>MPVAGSELQYLGQIQHILRCGVRKDDRTGTGTLSVFGMQARYSLRDEFPLLTTKRVFWKGVLEELLWFIKGSTNAKELSSKGVKIWDANGSRDFLDSLGFSTREEGDLGPVYGFQWRHFGAEYRDMESDYSGQGVDQLQRVIDTIKTNPDDRRIIMCAWNPRDLPLMALPPCHALCQFYVVNSELSCQLYQRSGDMGLGVPFNIASYALLTYMIAHITGLKPGDFIHTLGDAHIYLNHIEPLKIQL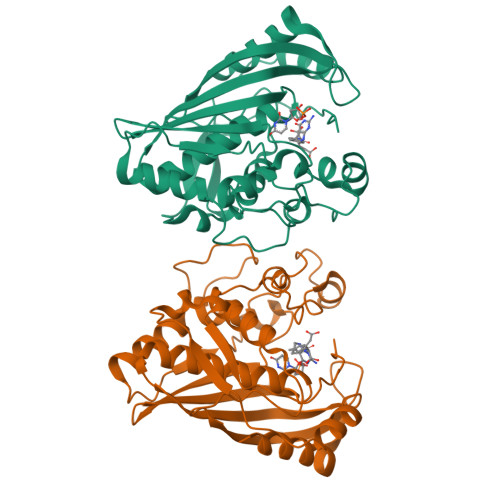QREPRPFPKLRILRKVEKIDDFKAEDFQIEGYNPHPTIKMEMAV[4x]>[2x]PGENLKPVDAMQCFDCHTQIEDMHTVGKHATVNCVHCHDATEHVETASSRRMGERPVTRMDLEACATCHTAQFNSFVEVRHESHP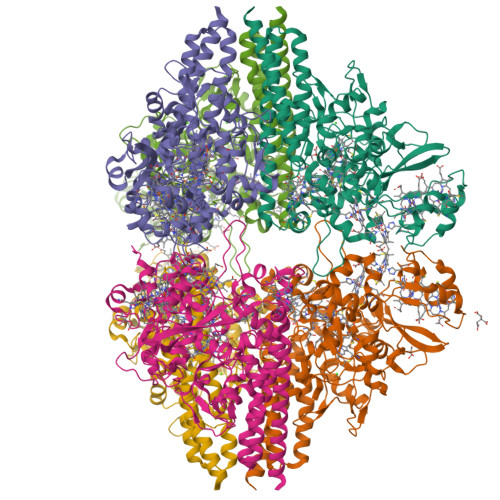RLEKATPTSRSPMFDKLIAGHGFAFEHAEPRSHAFMLVDHFVVDRAYGGRFQFKNWQKVTDGMGAVRGAWTVLTDADPESSDQRRFLSQTATAANPVCLNCKTQDHILDWAYMGDEHEAAKWSRTSEVVEFARDLNHPLNCFMCHDPHSAGPRVVRDGLINAVVDRGLGTYPHDPVKSEQQGMTKVTFQRGREDFRAIGLLDTADSNVMCAQCHVEYNCNPGYQLSDGSRVGMDDRRANHFFWANVFDYKEAAQEIDFFDFRHATTGAALPKLQHPEAETFWGSVHERNGVACADCHMPKVQLENGKVYTSHSQRTPRDMMGQACLNCHAEWTEDQALYAIDYIKNYTHGKIVKSEYWLAKMIDLFPVAKRAGVSEDVLNQARELHYDAHLYWEWWTAENSVGFHNPDQARESLMTSISKSKEAVSLLNDAIDAQVASR>TTHTSDFLKLNPSSGLWPASGL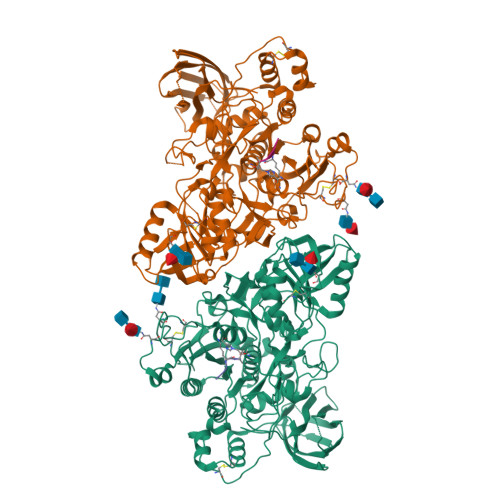GQDVIVAVLDSGIWPESASFQDDGMPEIPKRWKGICKPGTQFNASMCNRKLIGANYFNKGILANDPTVNITMNSARDTDGHGTHCASITAGNFAKGVSHFGYAPGTARGVAPRARLAVYKFSFNEGTFTSDLIAAMDQAVADGVDMISISYGYRFIPLYEDAISIASFGAMMKGVLVSASAGNRGPGIGSLNNGSPWILCVASGHTDRTFAGTLTLGNGLKIRGWSLFPARAFVRDSPVIYNKTLSDCSSEELLSQVENPENTIVICDDNGDFSDQMRIITRARLKAAIFISEDPGVFRSATFPNPGVVVNKKEGKQVINYVKNSVTPTATITFQETYLDTKPAPVVAASSARGPSRSYLGISKPDILAPGVLILAAYPPNVFATSIGTNILLSTDYILESGTSMAAPHAAGIAAMLKAAHPEWSPSAIRSAMMTTADPLDNTRKPIKDSDNNKAATPLDMGAGHVDPNRALDPGLVYDATPQDYVNLLCSLNFTEEQFKTIARSSASHNCSNPSADLNYPSFIALYSIEGNFTLLEQKFKRTVTNVGKGAATYKAKLKAPKNSTISVSPQILVFKNKNEKQSYTLTIRYIGDEGQSRNVGSITWVEQNGNHSVRSPIVTSPIIEVW[2x]>[3x]KPIEI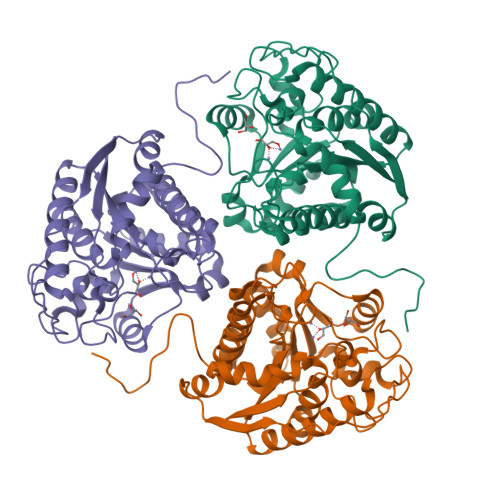IGAPFSKGQPRGGVEKGPAALRKAGLVEKLKETEYNVRDHGDLAFVDVPNDSPFQIVKNPRSVGKANEQLAAVVAETQKNGTISVVLGGDHSMAIGSISGHARVHPDLCVIWVDAHTDINTPLTTSSGNLCGQPVAFLLKELKGKFPDVPGFSWVTPCISAKDIVYIGLRDVDPGEHYIIKTLGIKYFSMTEVDKLGIGKVMEETFSYLLGRKKRPIHLSFDVDGLDPVFTPATGTPVVGGLSYREGLYITEEIYKTGLLSGLDIMEVNPTLGKTPEEVTRTVNTAVALTLSCFGTKREGNHKPETDYL>[20x]TPQNITDLCAEYHNTQIYTLNDKIFSYTESLAGKREMAIITFK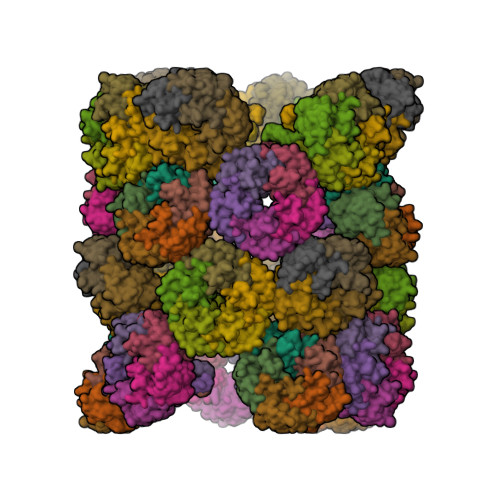NGAIFQVEVPGSQHIDSQKKAIERMKDTLRIAYLTEAKVEKLCVWNNKTPHAIAAISMANGVSALEKEVSALKEKVSALEF>GIDPFTTRPSSDLTAFREHFAKAKHIAIITGAGVSAESGVPTFRGPGGFWRKWQAQDLATPEAFSRDPSLVWEFYHYRREVMRSKMPNPAHLAIAECEARLGQQGRSVVIITQNIDELHHRAGSKHVYEIHGSLFKTRCMSCGEVKANHKSPICPALDGKGAPDPNTKEARIPVELLPRCERKSCNGLLRPHV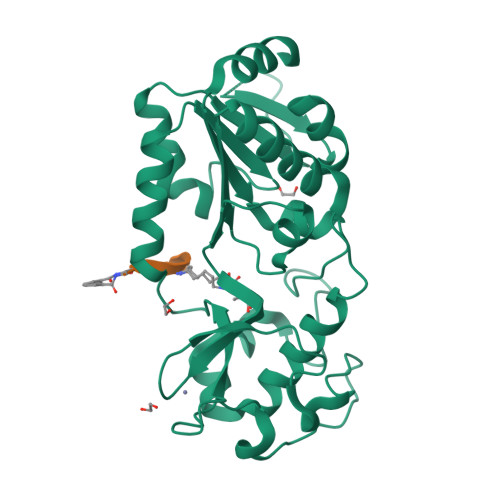VWFGETLDSDILTAVERELEKCDLCLVVGTSSIVYPAAMFAPQVASRGVPVAEFNMECTPATQRFKYHFEGPCGSTLPPALE[2x];> XGVLKEYGV>MKLTASLTLLTQALAVLGADTNSWKSRTIYFALTDRVARSASDNGGDGCGQLQDYCGGTFKGLEGKLDYIKGMGFDAIWITPVVQNSARGYHGYWASNLYATNSHYGTSDELKGLVNAAHGKGIYIMVDVVANHVGNGPLNEMQPAPLNQGSSYHPACGINYNDQHSIETCRVASDLPDLDTTDPKIRTLYKDWIKWLMSTYKFDGVRIDTVKHVEKDFWPDFAWASGSYTIGEVFSGDPNYVAGYSKLMGGLLNYPVYFPLNRFYQQQNSSQALVDMHNQIGSLVPDPTTLGTFLDNHDNPRFLSQKNDVSLFKNALTYVLLARGIPIVYYGSEQAYAGGGDPQNREDLWRSRFNTNSDMYKFFQALGGVRKSHGGLPGNDHVHLFVESDAYAWSRQDGAVMALTSNIGKGQQRQFCFFTQKNNKTWRGIFDGKTYTSGGDGKLCATVNNGEPIVFVAQ[2x]

Here, we describe the structure and function of three novel α-amylases from Cordyceps farinosa (CfAM), Rhizomucor pusillus (RpAM) and Thamnidium elegans (TeAM) with a higher stability and pH-tolerance with the potential to act as novel biocatalysts for various industrial processes. The sequence of all three enzymes groups them in the GH13 sub-family 1 along with, for example, the amylase from Aspergillus oryzae (also known as TAKA amylase). All three amylases have the classical domain structure with a central (β/α)8-barrel with the active site located on its C-terminal face, together with a small subdomain, inserted between the third strand and helix and a C-terminal β-sandwich. All three amylases have as their hallmark a shortened loop between β2/α3 and two shorter loops in subdomain B located between β3 and α4 of the central (β/α)8-barrel, compared to structures of other fungal amylases, e.g., TAKA-amylase.

For CfAM, there are two monomers in the asymmetric unit comprising residues 19 to 459 for chain A and 19 to 460 for chain B, which superpose with an r.m.s.d. of 0.3 Å. Two conserved disulphide bridges stabilize flexible loops in subdomains A and B. There is an additional disulphide bridge in CfAM, located in the C-terminal domain. In particular, CfAM shows the highest pH tolerance, retaining 70% of its activity at pH 8. Although all three amylases were co-crystallized with acarbose, a well-known inhibitor for amylases, a complex with acarbose bound was only obtained for TeAM and CfAM. As expected, the acarbose was found in the substrate binding cleft in each monomer of TeAM and CfAM, with the acarviosine unit sitting in subsites -1 and +1. The catalytic nucleophile D190/D192(CfAM/TeAM) is in a near attack conformation poised to react with the anomeric carbon, whilst the catalytic acid/base E214/E216(CfAM/TeAM) forms a hydrogen bond with the bridging nitrogen of the glycosidic bond with the 4-deoxyglucose in subsite +1. In CfAM, a secondary binding site in domain C was identified and modelled as maltose located at the edge of the β-sandwich. The glucose units are held in place mainly via hydrogen bonds without the usual stacking interactions with aromatic side chains. The additional binding site in this domain in CfAM strengthen the role of this domain in substrate binding. In addition, a new previously unobserved carbohydrate binding site was revealed in the C-terminal β-sandwich domain of CfAM, which might be important for the initial interaction with its polymeric substrate.> RLYWDDLKRKLSEKLDSTDFTSTIKLLNENSYVPREAGSQKDENLALYVENQFREFKLSKVWRDQHFVKIQVKDSAQNSVIIVDKNGRLVYLVENPGGYVAYSKAATVTGKLVHANFGTKKDFEDLYTPVNGSIVIVRAGKITFAEKVANAESLNAIGVLIYMDQTKFPIVNAELSFFGHAHLGTGDPYTPGFPSFNHTQFPPSRSSGLPNIPVQTISRAAAEKLFGNMEGDCPSDWKTDSTCRMVTSESKNVKLTVSNVLKEIKILNIFGVIKGFVEPDHYVVVGAQRDAWGPGAAKSGVGTALLLKLAQMFSDMVLKDGFQPSRSIIFASWSAGDFGSVGATEWLEGYLSSLHLKAFTYINLDKAVLGTSNFKVSASPLLYTLIEKTMQNVKHPVTGQFLYQDSNWASKVEKLTLDNAAFPFLAYSGIPAVSFCFCEDTDYPYLGTTMDTYKELIERIPELNKVARAAAEVAGQFVIKLTHDVELNLDYERYNSQLLSFVRDLNQYRADIKEMGLSLQWLYSARGDFF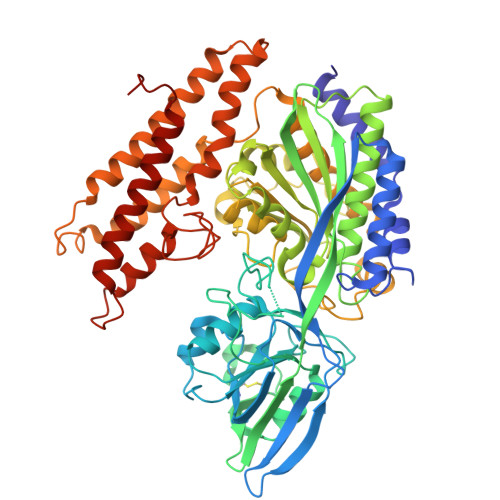RATSRLTTDFGNAEKTDRFVMKKLNDRVMRVEYHFLSPYVSPKESPFRHVFWGSGSHTLPALLENLKLRKQNNGAFNETLFRNQLALATWTIQGAANALSGDVWDIDNEF>[12x]MRGSHHHHHHGMASMAVSESQLKKMVSKYKYRDLTVRETVNVITLYKDLKPVLDSYV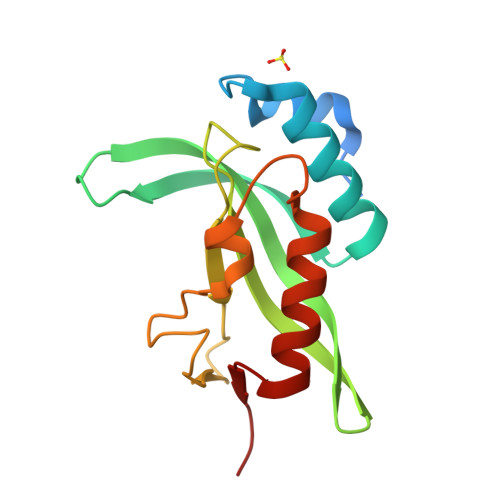FNDGSSRELMNLTGTIPVPYRGNTYNIPICLWLLDTYPYNPPICFVKPTSSMTIKTGKHVDANGKIYLPYLHEWKHPQSDLLGLIQVMIVVFGDEPPVFSRP>[4x]AFYKREMFDPAEKYKMDHRRRGIALIFNHERFFWHLTLPERRGTCADRDNLTRRFSDLGFEVKCFNDLKAEELLLKIHEVSTVSHADADCFVCVFLSHGEGNHIYAYDAKIEIQTLTGLFKGDKCHSLVGKPKIFIIQACRGNQHDVPVIPLDVVD;>AASVYTLPAGADFLMCYSVAEGYYSHRETVNGSWYIQDLCEMLGKYGSSLEFTELL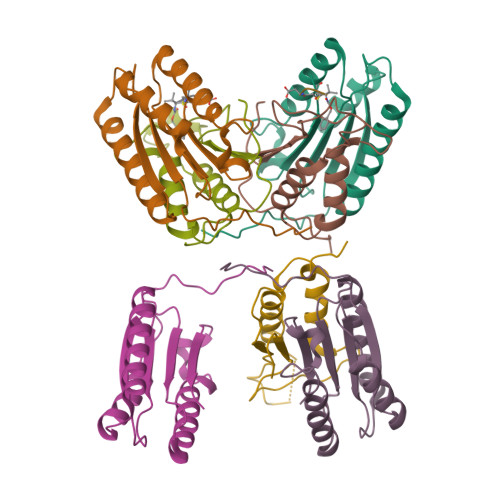TLVNRKVSQRRVDFCKDPSAIGKKQVPCFASMLTKKLHFFPKSN[4x]> AEIYNKDGNKVDLYGKAVGLHYFSKGNGENSYGGNGDMTYARLGFKGETQINSDLTGYGQWEYNFQG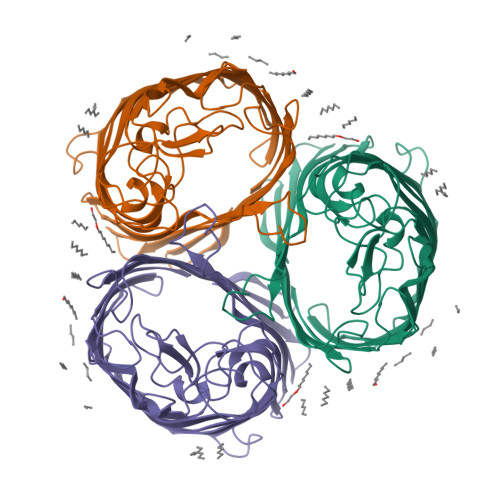NNSEGADAQTGNKTRLAFAGLKYADVGSFDYGRNYGVVYDALGYTDMLPEFDGDTAYSDDFFVGRVGGVATYRNSNFFGLVDGLNFAVQYLGKNERDTARRSNGDGVGGSISYEYEGFGIVGAYGAADRTNLQEAQPLGNGKKAEQWATGLKYDANNIYLAANYGETRNATPITNKFTNTSGFANKTQDVLLVAQYQFDFGLRPSIAYTKSKAKDVEGIGDVDLVNYFEVGATYYFNKNMSTYVDYIINQIDSDNKLGVGSDDTVAVGIVYQF>AIERTLSIIKPDGLEKGVIGKIISRFEEKGLKPVAIRLQHLSQAQAEGFYAVHKARPFFKDLVQFMISGPVVLMVLEGENAVLANRDIMGATNPAQAAEGTIRKDFAT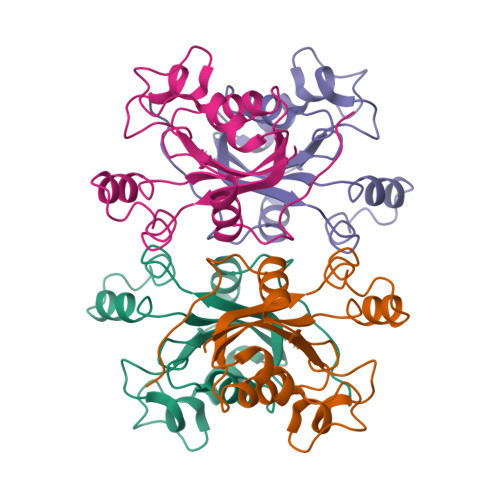SIDKNTVHGSDSLENAKIEIAYFFRETEIHSYPYQK[2x]> ASMTGNECPELQPPVHGKIEPSQAKYFFKDQVLVSCDTGYKVLKDNVEMDTFQIECLKDGTWSNKIPTCKIVDCRAPGELEHGLITFSTRNNLTTYKSEIKYSCQEPYYKMLNNNTGIYTCSAQGVWMNKVLGRSLPTCLPVCGLPKFSRKLMAR;> IFNGRPAQKGTTPWIAMLSHLNGQPFCGGSLLGSSWIVTAAHCLHQSLDPEDPTLRDSDLLSPSDFKIILGKHWRLRSDENEQHLGVKHTTLHPQYDPNTFENDVA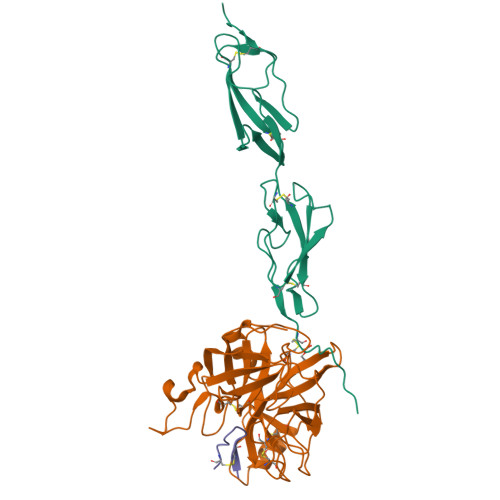LVELLESPVLNAFVMPICLPEGPQQEGAMVIVSGWGKQFLQRFPETLMEIEIPIVDHSTCQKAYAPLKKKVTRDMICAGEKEGGKDACAGDSGGPMVTLNRERGQWYLVGTVSWGDDCGKKDRYGVYSYIHHNKDWIQRVTGVRN;> GICSRSLPPICIPD>HMASMRISSLTLGLVDTNTYFIENDKAVILIDPSGESEKIIKKLNQINKPLKAILLTHAHFDHIGAVDDIVDRFDVPVYMHEAEFDFLKDPVKNGADKFKQYGLPIITSKVTPEKLNEGSTEIEGFKFNVLHTPGHSPGSLTYVFDEFAVVGDTLFNNGIGRTDLYKGDYETLVDSIQDKIFELEGDLPLFPGHGPYTTVDDEQLNPFLHG[4x]

Here we identify the bacterial esterases, GloB and FrmB, that activate carboxy ester prodrugs in Staphylococcus aureus. To establish the structural basis for FrmB and GloB substrate specificity and enable future structure-guided prodrug therapeutic design, we solved the three-dimensional structures of both S. aureus FrmB and GloB. FrmB and GloB have distinct ester substrate specificities, which are supported by the structures of their active sites. Additionally, the finding that mutation in either frmB or gloB is sufficient to confer POM-HEX resistance suggests that the two enzymes may work in concert to bioconvert POM-HEX into HEX.

GloB is predicted to be a type II glyoxalase and a member of the large metallo-β-lactamase protein superfamily (INTERPRO IPR001279). SaGloB hydrolyzes S-lactoylglutathione with a specific activity comparable to previously characterized microbial type II glyoxalases, but SaFrmB lacks appreciable glyoxalase activity. We also solved the structure of SaGloB to 1.65 Å, using selenomethionine (SeMet)-substituted GloB, and molecular replacement, using metallo-β-lactamase TTHA1623 from Thermus thermophilus as a search model. Four monomers of SaGloB are observed in the asymmetric unit with each displaying crystallographic symmetry. SaGloB exhibits the classic αβ/βα-fold that defines the metallo-β-lactamases, including glyoxalase II (Cameron et al., 1999; Honek, 2015; Stamp et al., 2010; Yamamura et al., 2009). Also consistent with previously observed GloB structures, SaGloB shows clear electron density for two zinc ions coordinated by six histidines and two aspartates. Density for a water molecule is also visible and appears to be coordinated by the two zinc ions, as observed for human glyoxalase II. On the opposite side of the active site, SaGloB has a 19-amino acid flexible loop, which is partially observed in the electron density. This loop is positioned such that it may cover the active site to sterically hinder substrate access. The GloB active site channel appears moderately wide, explaining why extensively branched substrates are not tolerated.>MSNHHHHHHHHHHENLYFQSMSGFLIPNAKFTSNNGFEFLLPYYWNIAPNFDATITPHYMERRGLQWQNEFRYLLAPGSGTMALDWLPNDRIYTGPDGTDKNATRWLYYWGHSGVMDQVWRFNINYTRVSDPAYFTDLTSQYGSTTDGYATQIFTAGYANENWNATLSSKQFQVFTAAGNSNAYRAQPQLDMNYYKNDVGPFDMHVYGQAAKFTSVNPTNPEASRFHIEPTVNLPLSNSWGSINTEAKLLATHYQQDIPASFADNASNPKLKDSVNRVLPQFKVDGKVVFDRSMDWATGFTQTLEPRAQYLYVPYRNQDDIYIYDTTLMQSDYSGLFRDRTYSGLDRIASANQVSTGLTSRIYDDARVERFNVSVGQIYYFSRSRTGNTEAIDNSNATGSLVWAGDTFWRINDQLGLKGGAQYDTRLGSLTLGNAIMEYRKDADRMIQLNYRYASPKYIQAAVPKVYNPDYQQGISQVGTTASWPIADRWAIVGAYYYDTKAKQPASQLVGLQYNTCCWAVNLGYERKITGWNAQGQTSKYDNKIGFNIELRGLSGGHSLGTAQMLNSGILPYQSAF[4x];>APNTSGFNLRGTTQVPTELQKLLLESSDPYGPLARSIRQQLRLNNVTIVDDAMRKDIPTLRIIGSSESQETVSI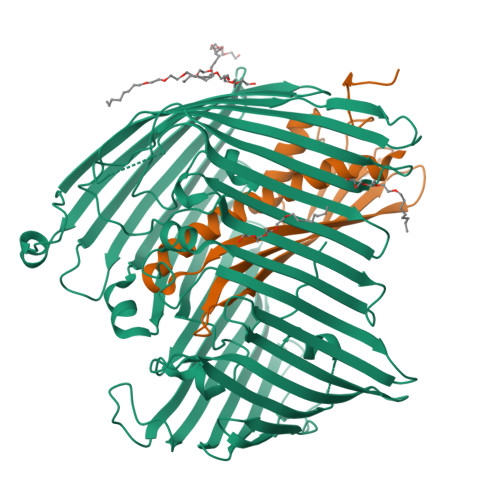FRNGVAAENQLVLHVQAQVLIPGHDIYPLQVNVFRTFFDNPLTALAKEAEAEVLRQEMREQAAQQLVRQLLTVHAAEVKNTQKNGDKPVSDANAAQGSTPTAVNETTLGEPAVSTSAKHHHHHH[4x]>GMDISLLKQVVQSTNKIALSTAVNNEADVKIVNFVWYEAQPDTLY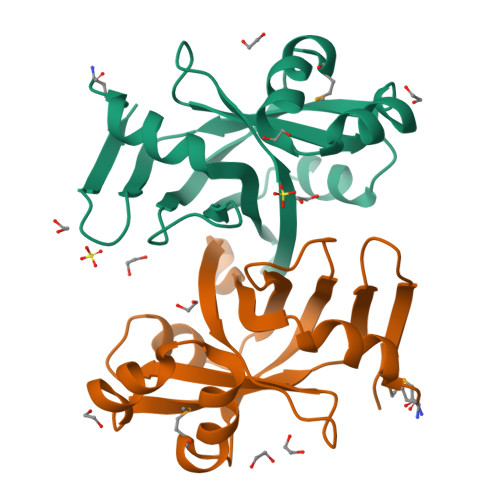FSSVKTSPALKVYDQNPDIAFITIPNDGTAGNPYLRAQHVKLQRSTKTMTDLLPQYLETVPNYQQVWDAIGSTLVVFELKLTDLFVDAGVGGEKQTLTFN[2x]>[2x]MHHHHHHYFSINDSKILSLQNKKNTLMDTSGYNAEVRVEGNVQLNPIFPFDFKLGSSGDDRGKVIVTQNENIVYNAMYESFSISFWIRINKWVSNLPGYTIIDSVKNNSGWSIGIISNFLVFTLKQNENSEQDINFSYDISKNAAGYNKWFFVTITTNMMGNMMIYINGKLIDTIKVKELTGINFSKTITFQMNKIPNTGLITSDSDNINMWIRDFYIFAKELDDKDINILFNSLQYTNVVKDYWGNDLRYDKEYYMINVNYMNRYMSKKGNGIVFNTRKNNNDFNEGYKIIIKRIRGNTNDTRVRGENVLYFNTTIDNKQYSLGMYKPSRNLGTDLVPLGALDQPMDEIRKYGSFIIQPCNTFDYYASQLFLSSNATTNRLGILSIGSYSFKLGDDYWFNHEYLIPVIKIEHYASLLESTSTHWVFVPAS

Botulinum neurotoxins (BoNTs) are a family of bacterial toxins produced by diverse strains of anaerobic clostridial bacteria. BoNTs are classified into seven major serotypes (BoNT/A–G). They are produced as ~150 kDa proteins, composed of a ~50 kDa light chain (LC) and a ~100 kDa heavy chain (HC). The HC contains two functional domains: the translocation domain on the N-terminal half (HN) and the receptor-binding domain on the C-terminal half (HC). BoNTs target neurons with exquisite specificity, which is achieved by recognizing two receptors in a “double-receptor” model.

The LC and HN of BoNT/DC are almost identical to the corresponding regions in BoNT/D, while its HC is most similar to BoNT/C1-HC. To identify the potential moiety on gangliosides recognized by BoNT/DC, we sought to determine the X-ray co-crystal structure of BoNT/DC-HC in complex with Sialyl-T. Co-crystallization of BoNT/DC-HC with Sialyl-T yielded crystals diffracting to 2.6 Å, with space group P41212. The complex contains two molecules per asymmetric unit (ASU), with well-defined electron density for Sialyl-T. Due to crystal contacts, Sialyl-T bound to chain A in the crystal is highly ordered, whereas the other Sialyl-T bound to chain B has much weaker electron density in the parts of Sialyl-T not interacting with BoNT/DC-HC. No significant differences were observed in the interactions between Sialyl-T and BoNT/DC-HC between the two Sialyl-T molecules, so from here on all data we report are based on the well-defined Sialyl-T molecule bound to chain A. The structure revealed that Sialyl-T binds to BoNT/DC-HC with a total of seven hydrogen bonds, all originating from the terminal sialic acid. There are two hydrogen bonds to S1242, one each to N1114, Y1115, I1240, and S1275. An additional hydrogen bond is formed with Y1243 via a bridging water molecule. The location of the Sialyl-T binding site in BoNT/DC is homologous to the well-defined GBS site in other BoNTs. The major difference is that this site in BoNT/DC forms contacts with only the sialic acid, but not the Gal-GalNAc, whereas the conserved GBS site in other BoNTs interacts with all three moieties. Essentially, the GBS in BoNT/DC has “degenerated” into a sialic acid-binding site.1-(5-CHLORO-2,4-DIMETHOXYPHENYL)-3-(5-CYANOPYRAZIN-2-YL)UREA | C14 H12 Cl N5 O3 | 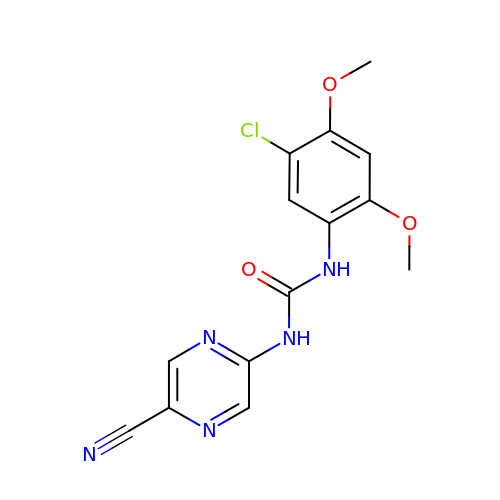URQYPXQXSVUVRG-UHFFFAOYSA-N> DWYHRIDHTVLLGALPLKNMTRRLVLDENVR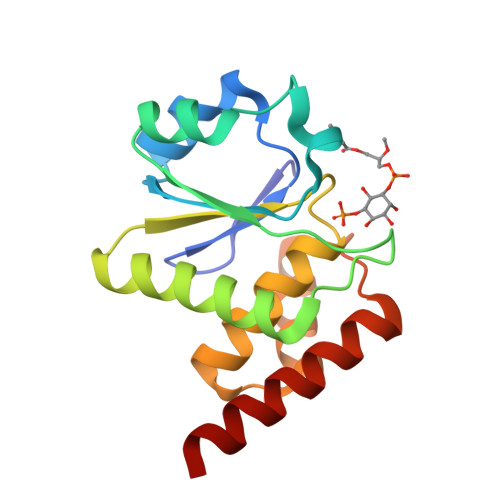GVITMNEEYETRFLCNTSKEWKKAGVEQLRLSTVDMTGVPTLANLHKGVQFALKYQALGQCVYVHSKAGRSRSATMVAAYLIQVHNWSPEEAIEAIAKIRSHISIRPSQLEVLKEFHKEITARAA> GAGCAGACATGACG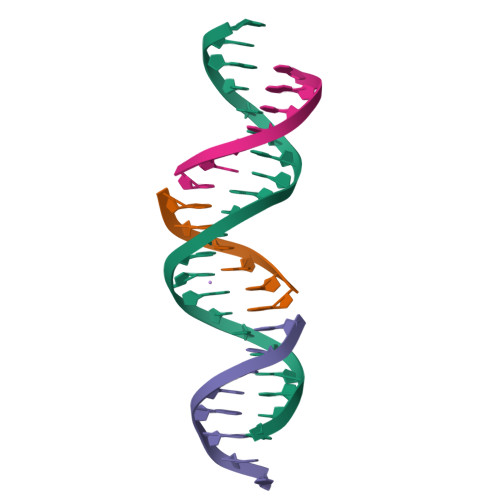TCACTCA;> ACGTCA;> TCTGAGTG;> TGTCTGC In this context, we recently proposed a lanthanide-based molecule, named the crystallophore (Tb-Xo4). Tb-Xo4 is a cationic complex with nucleating and phasing properties. In particular, we show that Tb-Xo4 may provide different crystal forms of a single protein and correct the often-encountered defects in crystalline order that may result in low-resolution data as well as twinning. We prove that, beyond these crystallization properties, Tb-Xo4 is one of the most efficient phasing tools compatible with serial crystallography approaches.

We successfully obtained different crystallization hits for this protein mixture in the presence of 10 mM Tb-Xo4. In the absence of the crystallophore, no crystal was obtained in the same conditions. Because of the presence of multiple proteins in this fraction, it was quite difficult to assign the protein identity to the crystal by using mass spectrometry. III-absorption edge to maximize the terbium anomalous contribution. Among the recorded data sets, one presented diffraction at 2 Å resolution and a significant amount of anomalous signal. The protein was sequenced using the electron density, and a search for the sequence in the genomic database of M. thermolithotrophicus matched with adenylate kinase (AdkA), a trimeric enzyme that catalyses the interconversion of adenine-type nucleotides. By providing the full sequence, the automatic building completed the model at 95%. Finally, the straightforward ab initio phasing of the protein AdkA is an additional example of the unmatched phasing power of Tb-Xo4.

>MKNKLVVVTGVPGVGGTTITQKAMEKLSEEGINYKMVNFGTVMFEVAQEENLVEDRDQMRKLDPDTQKRIQKLAGRKIAEMVKESPVVVDTHSTIKTPKGYLPGLPVWVLNELNPDIIIVVETSGDEILIRRLNDETRNRDLETTAGIEEHQIMNRAAAMTYGVLTGATVKIIQNKNNLLDYAVEELISVLR[3x]3-{[(4-methylphenyl)carbamoyl]amino}benzoic 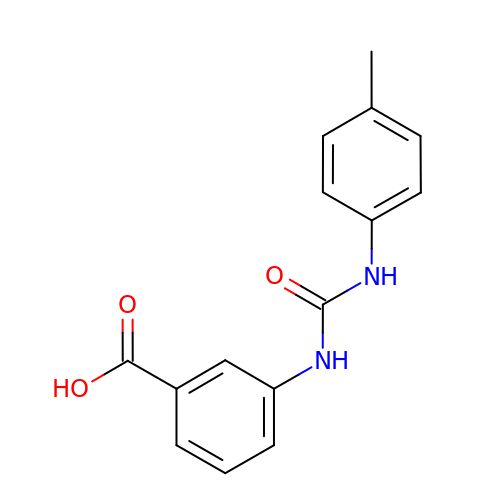acid | C15 H14 N2 O3 | TYCRWVKJQQIRNE-UHFFFAOYSA-N(6~{R})-7-thia-2-azatricyclo[6.3.1.0^{4,12}]dodeca-1(11),3,8(12),9-tetraene-6-carboxylic acid | 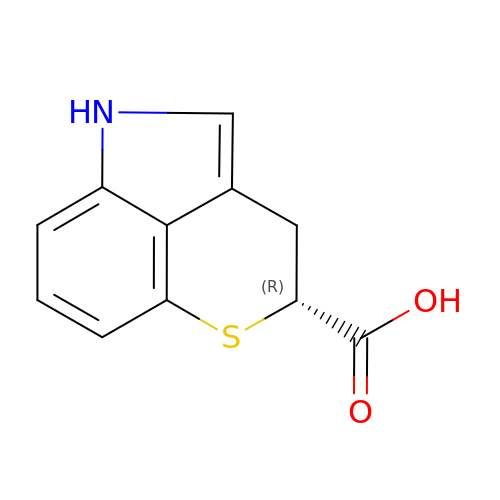C11 H9 N O2 S | IBFALAJQGUDUBZ-SECBINFHSA-N>[3x]GSHMSYNNIPAGKDAPNDIYVIIEIPANAAPIKYEIDKDSDALFVDRFMGTAMFYPANYGYVPNTLSEDGDPL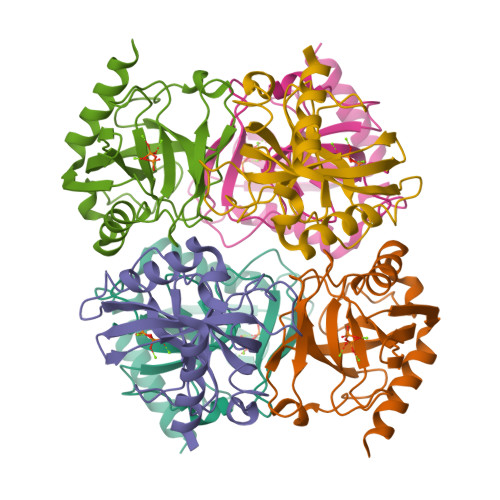DVLVVTPYPVAAGSVIRCRPVGKLNMEDDGGIDAKLIAVPHEKLSPLYKDVKEYTDLPQLLINQVEHFFSHYKDLEPGRWVKISGWEGADVAKAEVIKAIEAAK> MGDNLTD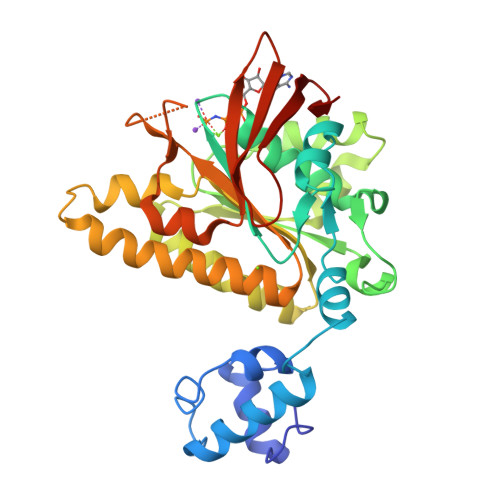LPGVGPSTAEKLVEAGYIDFMKIATATVGELTDIEGISEKAAAKMIMGARDLCDLGFKSGIDLLKQRSTVWKLSTSSSELDSVLGGGLESQSVTEFAGVFGSGKTQIMHQSCVNLQNPEFLFYDEEAVSKGEVAQPKAVYIDTDGTFRPERIMQMAEHAGIDGQTVLDNTFVARAYNSDMQMLFAEKIEDLIQEGNNIKLVVIDSLTSTFRNEYTGRGKLAERQQKLGRHMATLNKLADLFNCVVLVTNQVSAKPDAFFGMAEQAIGGHIVGHAATFRFFVRKGKGDKRVAKLYDSPHLPDAEAIFRITEKGIQD>[2x]MAHHHHHHMGGDVTFSLTKTRDTFADWFDAIMDAAELVDRRYPVKGCVVFRPYGFFMENAIMRLCEEEYAKVGISQILFPTVIPESFLKKESDHIKGFEAECFWVEKGGLQPLEERLALRPTSETAIYSMFSKWVRSYKDLPLKIHQTCTIFRHETKNTKPLIRVREIHWNEAHCCHATAEDAVSQLSDYWKVIDTIFSDELCFKGQKLRRVCWDRFPGADYSEVSDVVMPCGRVLQTAGIHNLGQRFSST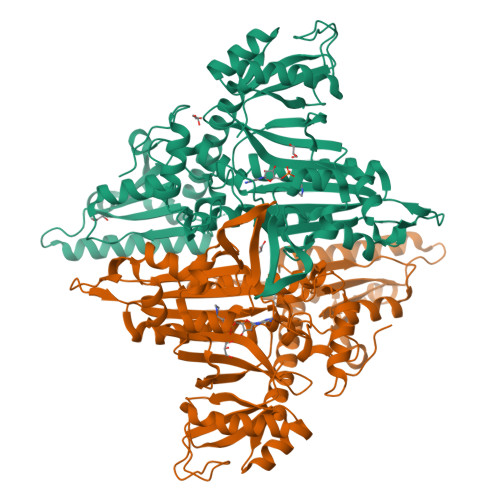FDILYANKANESVHPYLTCAGISTRVLACALSIHGDSGGLVLPPLIAPIHVVIIPIGCGKKNNQESDQQVLGKVNEIADTLKSKLGLRVSIDDDFSKSMGDKLYYYELKGVPLRIEVGQRDLANGQCIVVPRDVGKDQKRVIPITEVMKVSSHTTENHELVVKNVIKDELDAYKARLKEKAFAFHNSMVTNCKSFDEIVACIENKGGLARFPFYTTEADGEVWDKKLKDACSAEIRGHNPDENVLPGEVCALSGKPAVCYMYCAKSY>ADINHGENVFTANCSACHAGG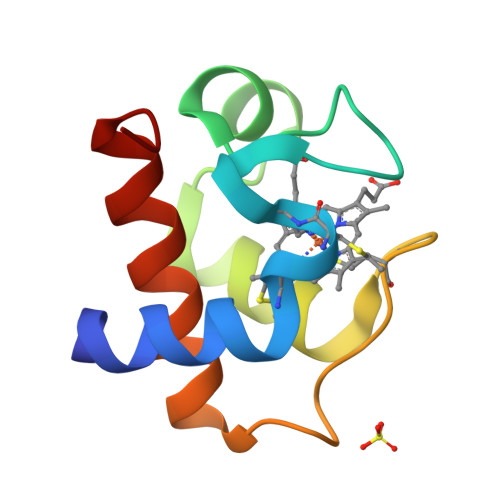NNVIMPEKTLQKDALSTNQMNSVGAITYQVTNGKNAMPAFGGRLSDDDIEDVASFVLSQSEKSWN[6x]3-(1,3,7-TRIHYDRO-9-D-RIBITYL-2,6,8-PURINETRIONE-7-YL) 1,1 DIFLUOROPENTANE-1-PHOSPHATE 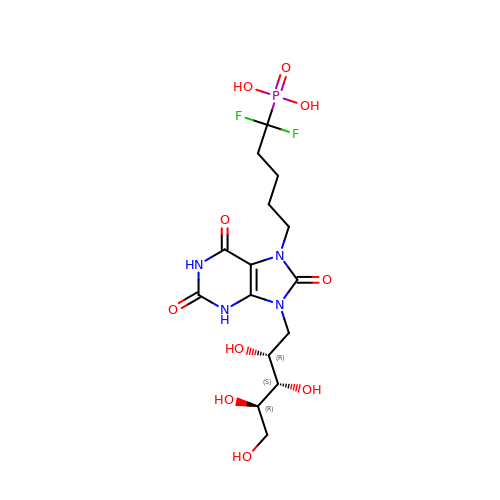| C15 H23 F2 N4 O10 P | ZBEBHCIQAVPUSI-MRTMQBJTSA-N> MQASQFSAQVLDWYDKYGRKTLPWQIDKTPYKVWLSEVMLQQTQVATVIPYFERFMARFPTVTDLANAPLDEVLHLWTGLGYYARAR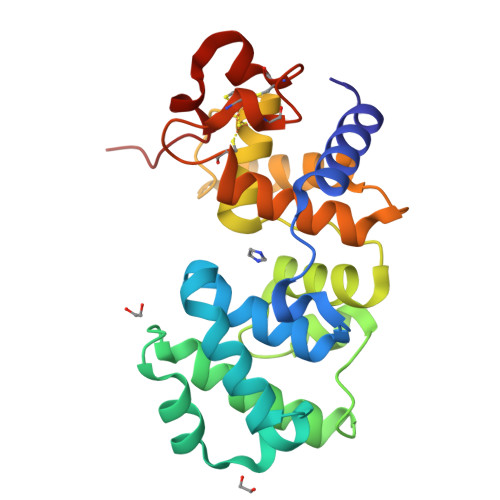NLHKAAQQVATLHGGKFPETFEEVAALPGVGRSTAGAILSLSLGKHFPILDGNVARVLARCYAVSGWPGKKEVENKLWSLSEQVTPAVGVERFNQAMMDLGAMICTRSKPKCSLCPLQNGCIAAANNSWALYPGKKPK> ASNLVCYYDSSSYTREGLGKLLNPDLEIALQFCSHLVYGYAGLRGENLQAYSMNENLDIYKHQFSEVTSLKRKYPHLKVLLSVGGDHDIDPDHPNKYIDLLEGEKVRQIGFIRSAYELVKTYGFDGLDLAYQFPKNKPRKVHGDLGLAWKSIKKLFTGDFIVDPHAALHKEQFTALVRDVKDSLRADGFLLSLTVLPNVNSTWYFDIPALNGLVDFVNLATFDFLTPARNPEEADYSAPI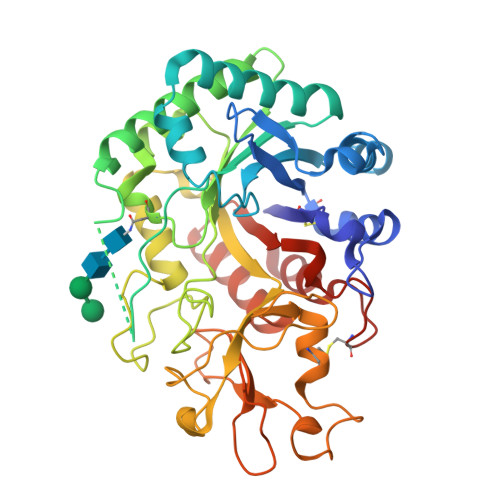YHPDGSKDRLAHLNADFQVEYWLSQGFPSNKINLGVATYGNAWKLTKDSGLEGVPVVPETSGPAPEGFQSQKPGLLSYAEICGKLSNPQNQFLKGNESPLRRVSDPTKRFGGIAYRPVDGQITEGIWVSYDDPDSASNKAAYARVKNLGGVALFDLSYDDFRGQCSGDKYPILRAIKYRL> MAKVEQVLSLEPQHELKFRGPFTDVVTTNLKLGNPTDRNVCFKVKTTVPRRYCVRPNSGVIDAGASLNVSVMLQPFDYDPNEKSKHKFMVQSMFAPPDTSDMEAVWKEAKPEDLMDSKLRCVFEL;> SEDSFFSATE

Mitoguardin-2 (MIGA2), a mitochondrial outer membrane protein, forms the ERMCS in higher eukaryotic cells. Mammalian MIGA2 has several distinct domains: a mitochondrial targeting transmembrane domain (TM) at the N-terminus, a coiled-coil domain, the FFAT motif, and a large C-terminal LD targeting domain. Here, we report the crystal structures of the MIGA2 LD targeting domain and the major sperm protein (MSP) domain of VAPB bound to the phosphorylated FFAT motif of MIGA2. MIGA2 (yellow orange) forms a complex with VAPB (gray) via the phosphorylated FFAT motif and then transfers lipids between the membranes by extracting and interiorizing lipids into its large hydrophobic cavity.

To answer this question, we solved the crystal structure of mouse VAPB MSP domain bound a phosphorylated FFAT peptide from mMIGA2 (residues 289–298, referred to as mMIGA2pFFAT) at 1.68 Å resolution. The overall structure of the mVAPB-mMIGA2pFFAT complex highly resembles that of VAPA-ORP1 (rmsd of 0.74 Å over 108 Cα) and VAPA-STARD3 (rmsd of 0.81 Å over 112 Cα), which possess a conventional and a single phosphorylated FFAT motif, respectively. Overall, the extended structure of mMIGA2pFFAT peptide binds across the center of mVAPB. The phosphorylated S292 residue forms an ionic bond with the side chain of a conserved K87 residue of mVAPB and also associates with the K118 residue of mVAPB via a water molecule. To test whether these residues are genuinely responsible for mVAPB interactions with mMIGA2pFFAT, we generated mutants (K43L/K45L and K87L/K118L) of mVAPB and measured their dissociation constants using ITC. While wild-type mVAPB showed a dissociation constant (Kd) of 1.7 ± 0.2 μM for mMIGA2pFFAT, the binding affinities of K87L/K118L and K43L/K45L mutants were 3- and 5-fold lower than that of wild type mVAPB, respectively. ITC measurements demonstrated that wild-type mMIGA2275–570 could not interact with mVAPB, whereas the S292E and S295D phosphorylation mimic mutants of mMIGA2275–570 showed binding affinities (Kd) of 26.4 ± 6.8 and 8.1 ± 1.5 μM, respectively. The S292E and S295D double mutations synergistically increased the binding affinity to 2.5 ± 0.3 μM, suggesting that both phosphorylations are needed for association with VAPB. In this study, we showed that phosphorylations at both S292 and S295 of mouse MIGA2 FFAT motif are required for its tight interaction with the VAPB using structural and biochemical analyses. The result suggests that the phosphorylation-induced MIGA2-VAPB interaction enhances the lipid transfer rate when both proteins are tethered.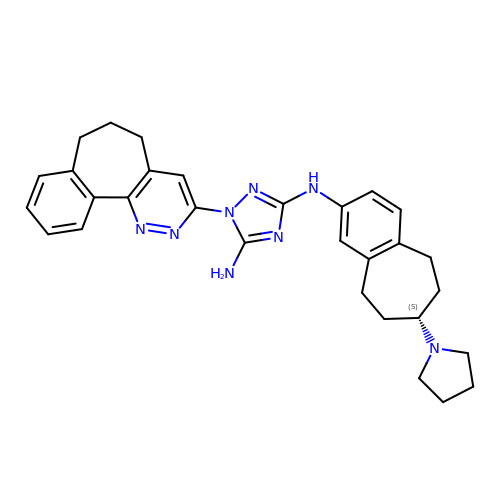1-(3,4-diazatricyclo[9.4.0.0^{2,7}]pentadeca-1(11),2(7),3,5,12,14-hexaen-5-yl)-~{N}3-[(7~{S})-7-pyrrolidin-1-yl-6,7,8,9-tetrahydro-5~{H}-benzo[7]annulen-3-yl]-1,2,4-triazole-3,5-diamine | C30 H34 N8 | KXMZDGSRSGHMMK-VWLOTQADSA-N> ATEATNATNNQSTQVSQATSQPINFQVQKDGSSEKSHMDDYMQHPGKVIKQNNKYYFQTVLNNASFWKEYKFYNANNQELATTVVNDNKKADTRTINV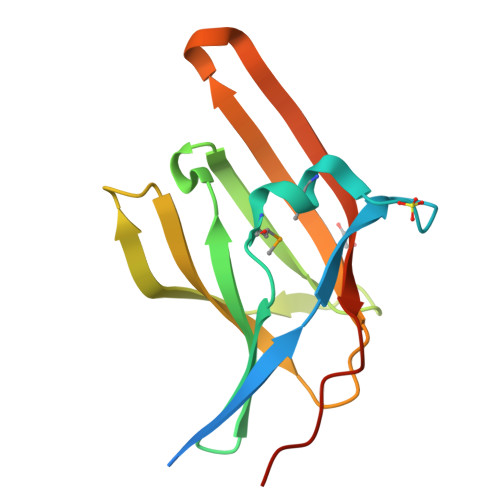AVEPGYKSLTTKVHIVVPQINYNHRYTTHLEFEKAIPTLADAAK> GEMDQDFDSLLLGFNDSDSVQKDPTV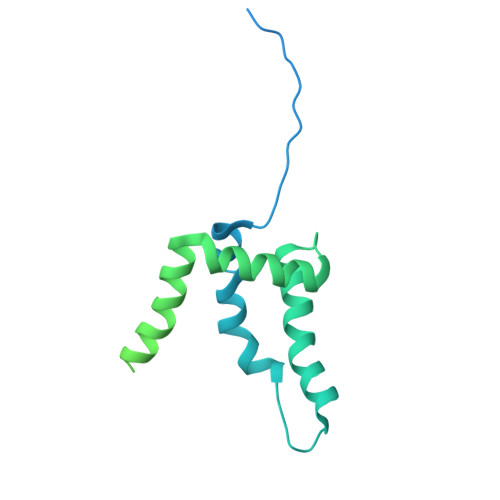PNGLDGSVVDPTIADPTAITARKRRPQVKLTAEKLLSDKGLPYVLKNAHKRIRISSKKNSYDNLSNIIQFYQLWAHELFPKAKFKDFMKICQTVGKTDPVLREYRVSLFRDEMGMSFDVGTRETGQDLERQSPMVEEHVTSAEERPIVADSFAQDKRNVNNVDYDNDEDDDIYHLSYRNRRGRVLDERGNNETVLNNVVPPKEDLDALLKTFRVQGPVGLEENEKKLLLGWLDAHRKMEKGSMTEEDVQLIQSLEEWEMNDIEGQHTHYDLLPGGDEFGVDQDELDAMKEMGF>MVRRTKEEAQETRAQIIEAAERAFYKRGVARTTLADIAELAGVTRGAIYWHFNNKAELVQALLDSLHETHDHLARASESEDEVDPLGCMRKLLLQVFNELVLDARTRRINEILHHKCEFTDDMCEIRQQRQSAVLDCHKGITLALANAVRRGQLPGELDAERAAVAMFAYVDGLIRRWLLLPDSVDLLGDVEKWVDTGLDMLRLSPALRK[2x]

TtgR is a multidrug binding repressor that negatively controls the transcription of the ttgABC operon as well as its own expression. TtgR belongs to the TetR family of proteins, which are characterized by a conserved DNA binding domain but variable ligand binding domain. A TtgR monomer consists of nine alpha helices forming two distinct domains. The DNA binding domain consists of α1–α3 (residues 1–53) while the ligand-binding domain consists of α4–α9 (residues 54–210), with an angle of approximately 80° between the two domains.

The structure of TtgR in complex with chloramphenicol was determined using selenomethionine substituted crystals and multiple-wavelength anomalous diffraction (MAD) methods and all subsequent structures were determined by molecular replacement method using the TtgR/chloramphenicol structure without the ligand as a starting model. The structure of TtgR in complex with chloramphenicol was also determined at 2.7 Å resolution. The TtgR structure is almost identical to that of TtgR in complex with tetracycline. Chloramphenicol is situated similarly to tetracycline and utilizes the general hydrophobic environment of the side walls with little specific interactions. In the case of quercetin, naringenin, tetracycline, chloramphenicol, as well as additional phloretin molecules, binding occurs vertically in the binding pocket with little specific interactions. This binding site is broader, more exposed, and contains less specific interactions. We therefore term this site the general binding site, which most probably contributes to the versatility of TtgR's ligand binding property.>[4x]ATTGTQGYTVVKNDWKKAVKQLQDGLKDNSIGKITVSFNDGV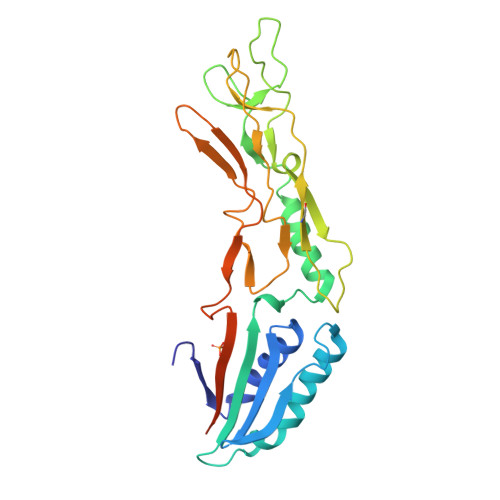VGEVAPKSANKKADRDAAAEKLYNLVNTQLDKLGDGDYVDFSVDYNLENKIITNQADAEAIVTKLNSLNEKTLIDIATKDTFGMVSKTQDSEGKNVAATKALKVKDVATFGLKSGGSEDTGYVVEMKAGAVEDKYGKVGDSTAGIAINLPSTGLEYAGKGTTIDFNKTLKVDVTGGSTPSAVAVSGFVTKDDTDLAKSGTINVRVINAKEESIDIDASSYHMSLEHHHHHH> 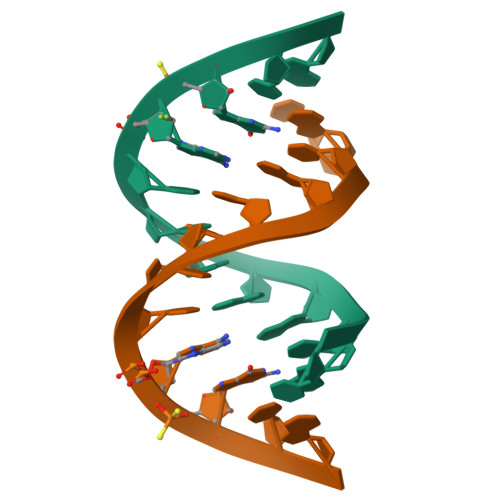CGCGAAUUXXCG>MQNHTAVNTAQAIILRDLVDALLFEDIAGIVSNSEITKENGQTLLIYERETQQIKIPVYFSALNMFRYESSQPITIEGRVSKQPLTAAEFWQTIANMNCDLSHEWEVARVEEGLTTAATQLAKQLSELDLASHPFVMSEQFASLKDRPFHPLAKEKRGLREADYQVYQAELNQSFPLMVAAVKKTHMIHGDTANIDELENLTVPIKEQATDMLNDQGLSIDDYVLFPVHPWQYQHILPNVFATEISEKLVVLLPLKFGDYLSSSSMRSLIDIGAPYNHVKVPFAMQSLGALRLTPTRYMKNGEQAEQLLRQLIEKDEALAKYVMVCDETAWWSYMGQDNDIFK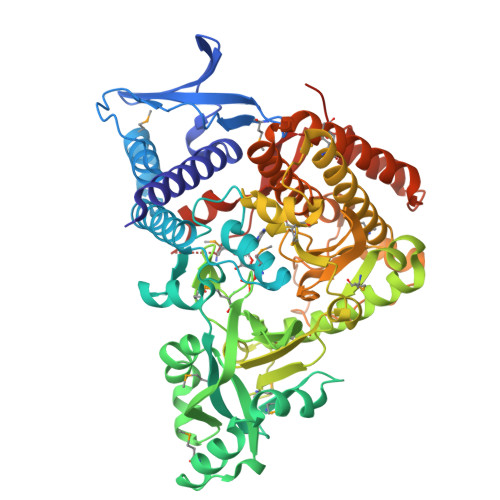DQLGHLTVQLRKYPEVLAKNDTQQLVSMAALAANDRTLYQMICGKDNISKNDVMTLFEDIAQVFLKVTLSFMQYGALPELHGQNILLSFEDGRVQKCVLRDHDTVRIYKPWLTAHQLSLPKYVVREDTPNTLINEDLETFFAYFQTLAVSVNLYAIIDAIQDLFGVSEHELMSLLKQILKNEVATISWVTTDQLAVRHILFDKQTWPFKQILLPLLYQRDSGGGSMPSGLTTVPNPMVTYDHHHHHH[2x]>ADSVNGAKIFSANCASCHAGGKNLVQAQKTLKKADLEKYGMYSAEAIIAQVTNGKNAHPAFKGRLKPEQIEDVAAYVLGKADADWK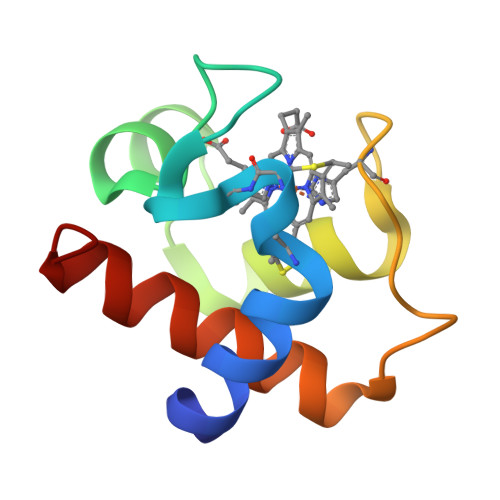[2x]> MATPSMMPQWSYMHIAGQDASEYLSPGLVQFARATDTYFSLGNKFRNPTVAPTHDVTTDRSQRLTLRFVPVDREDTAYSYKVRFTLAVGDNRVLDMASTYFDIRGVLDRGPSFKPYSGTAYNSLAPKTAPNPCEWKDNNKIKVRGQAPFIGTNINKDNGIQIGTDTTNQPIYADKTYQPEPQVGQTQWNSEVGAAQKVAGRVLKDTTPMLPCYGSYAKPTNEKGGQASLITNGTDQTLTSDVNLQFFALPSTPNEPKAVLYAENVSIEAPDTHLVYKPDVAQGTISSADLLTQQAAPNRPNYIGFRDNFIGLMYYNSTGNMGVLAGQASQLNAVVDLQDRNTELSYQLMLDALGDRSRYFSMWNQAVDSYDPDVRIIENHGVEDELPNYCFPLGGSAATDTYSGIKANGQTWTADDNYADRGAEIESGNIFAMEINLAANLWRSFLYSNVALYLPDSYKITPDNITLPENKNTYAYMNGRVAVPSALDTYVNIGARWSPDPMDNVNPFNHHRNAGLRYRSMLLGNGRYVPFHIQVPQKFFAIKNLLLLPGSYTYEWNFRKDVNMILQSSLGNDLRVDGASVRFDSINLYANFFPMAHNTASTLEAMLRNDTNDQSFNDYLCAANMLYPIPSNATSVPISIPSRNWAAFRGWSFTRLKTKETPSLGSGFDPYFTYSGSVPYLDGTFYLNHTFKKVSIMFDSSVSWPGNDRLLTPNEFEIKRTVDGEGYNVAQCNMTKDWFLIQMLSHYNIGYQGFYVPESYKDRMYSFFRNFQPMSRQVVNTTTYKEYQNVTLPFQHNNSGFVGYMGPTMREGQAYPANYPYPLIGQTAVPSLTQKKFLCDR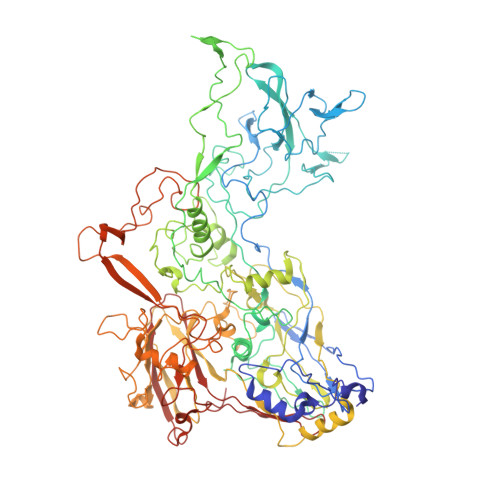TMWRIPFSSNFMSMGALTDLGQNMLYANSAHALDMTFEVDPMDEPTLLYVLFEVFDVVRIHQPHRGVIEAVYLRTPFSAGNATT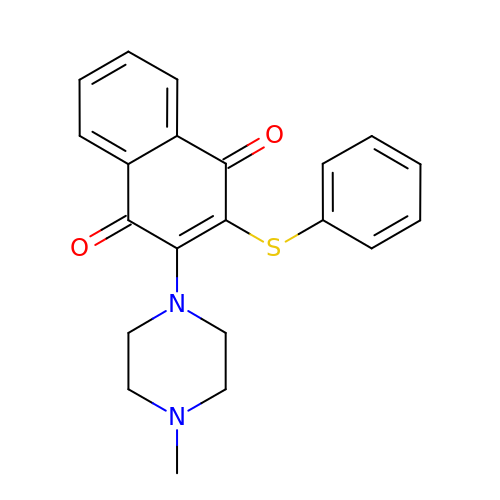2-(4-methylpiperazin-1-yl)-3-(phenylsulfanyl)naphthalene-1,4-dione | C21 H20 N2 O2 S | MJTBKNZEOWNOFN-UHFFFAOYSA-N>GVSLRKAERLRAELLDLKAGGFSIRNQKGEQVFRLAFRSGALDLDSCSRDGALLGCSLTADGLPLHFFIQTVRPKDTVMCYRVRWEEAAPGRAVEHAMFLGDAAAHWYGGAEMRTQHWPIRLDGQQEPQPFVTSDVYSSDAAFGGILERYWLSSRAAAIKVNDSVPFHLGWNSTERSLRLQARYHDTPYKPPAGRAAAPELSYRVCVGSDVTSIHKYMVRRYFNKPSRVPAPEAFRDPIWSTWALYGRAVDQDKVLRFAQQIRLHHFNSSHLEIDDMYTPAYGDFDFDEVKFPNASDMFRRLRDAGFRVTLWVHPFVNYNSSRFGEGVERELFVREPTGRLPALVRWWNGIGAVLDFTHPKARDWFQGHLRRLRSRYSVASFKFDAGEVSYLPRDFSTYRPLPDPSVWSRRYTEMALPFFSLAEVRVGYQSQNISCFFRLVDRDSVWGYDLGLRSLIPAVLTVSMLGYPFILPDMVGGNAVPQRTAGGDVPERELYIRWLEVAAFMPAMQFSIPPWRYDAEVVAIAQKFAALRASLVAPLLLELAGEVTDTGDPIVRPLWWIAP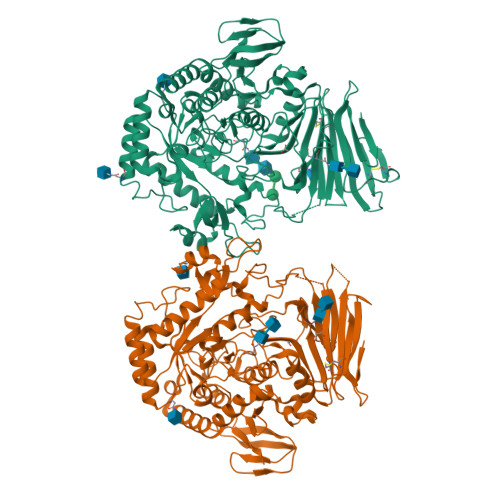GDETAHRIDSQFLIGDTLLVAPVLEPGKQERDVYLPAGKWRSYKGELFDKTPVLLTDYPVDLDEIAYFTWAS[4x]>[2x]APLAPCQNHHCKHGKVCELDENNTPMC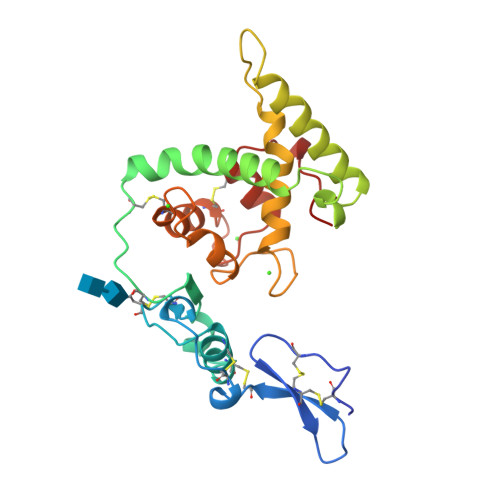VCQDPTSCPAPIGEFEKVCSNDNKTFDSSCHFFATKCTLEGTKKGHKLHLDYIGPCKYIPPCLDSELTEFPLRMRDWLKNVLVTLYERDEDNNLLTEKQKLRVKKIHENEKRLEAGDHPEKNYNMYIFPVHWQFGQLDQHPIDGYLSHTELAPLRAPLIPMEHCTTRFFETCDLDNDKYIALDEWAGCFGIKQKDIDKDLVI Using genome-wide transcriptional and functional analyses combined with structural and population genetics studies, we conclusively demonstrated that a single amino acid change in the binding pocket of the glutathione-s-transferase epsilon 2 (GSTe2) gene, coupled with increased transcription, confers a high level of DDT resistance and also cross-resistance to pyrethroids in the major African malaria vector An. funestus. The topology of GSTe2 indicates that the 221 amino acids of the An. funestus GSTe2 (afGSTe2) are divided into two distinct domains similar to that of An. gambiae (92% similarity between the two species, with a difference of 20 amino acids). The active site is located in a deep cleft formed at the interface of the two domains, specifically by the interaction of H1 and H3 from the N-terminal domain and H4, H6 and H8 from the C-terminal domain. The active site of GSTe2 can be divided into two sub-sites.

To identify the structural changes responsible for the higher activity in the resistant GSTe2 Benin allele (119 F), its X-ray three-dimensional structure was determined and analyzed in comparison with that of a L119-GSTe2 susceptible allele cloned from Uganda (UG-GSTe2). Overall, the structure of BN-GSTe2 and UG-GSTe2 are very similar. However, significant local differences can be observed between the alleles at the C-terminal ends of H4 (containing the L119F mutation; residues from 113 to 128) and H8 (residues from 213 to 220). These differences can be described as a concerted movement of the BN-GSTe2 H4 and H8 helices with respect to those of UG-GSTe2, which opens the active site cleft. Leu119 normally forms part of the solvent-inaccessible hydrophobic core that stabilizes the conformation of helices H4, H5 and H8 of Uganda-GSTe2. However, to accommodate the bulkier Phe119 side chain in the Benin-GSTe2 structure, the N-terminal end of H4 has a dramatic bend, which increases the size of the H-site in comparison to the UG allele, where the cavity is tighter. The H-site surface representation of both proteins with a bound GSH confirms that the resistant BN allele has a larger putative DDT cavity than the susceptible UG allele. An assessment of the DDT dehydrochlorinase activity of the recombinant 119 F resistant enzyme (Benin) and that of susceptible L119 revealed that the 119 F allele is 3.4 times more efficient at metabolizing DDT (82.9% DDT depletion after 1 hr reaction in the presence of the cofactor glutathione (GSH); P < 0.001) than the L119 allele (24.4% depletion). This is confirmed by their respective kinetic parameters, with the 119 F allele having a higher catalytic efficiency (kcat/Km ratio) for DDT (316.3 μM−1.s−1 vs 92.0 μM−1.s−1). Overall, these structural analyses demonstrate that the L119F mutation is the causative mutation that confers DDT resistance.

>[4x]SHMTKLVLYTLHLSPPCRAVELTAKALGLELEQKNINLLAGDHLTPEFMKLNPQHTIPVLDDDGTIITESHAIMIYLVTKYGKDDTLYPKDPVQQARVNAALHFESGVLFARMRFIFERIFFYGKSDIPEDRVEYVQKSYRLLEDTLKDDFVAGSKMTIADFSCISTISSIMGVVPLEQSEHPRIYEWIDRLKQLPYYEEANGGGGTDLGKFVLAKKEENAKA>[4x]MPLNRTLSMSSLPGLEDWEDEFDLENAVLFEVAWEVANKVGGIYTVLQTKAKVTGDEWGDNYFLVGPYTEQGVRTQVELLEAPTPALKRTLDSMNSKGCKVYFGRWLIEGGPLVVLLDVGASAWALERWKGELWDTCNIGVPWYDREANDAVLFGFLTTWFLGEFLAQSEEKPHVVAHFHEWLAGVGLCLCRARRLPVATIFTTHATLLGRYLCAGAVDFYNNLENFNVDKEAGERQIYHRYCMERAAAHCAHVFTTVSQITAIEAQHLLKRKP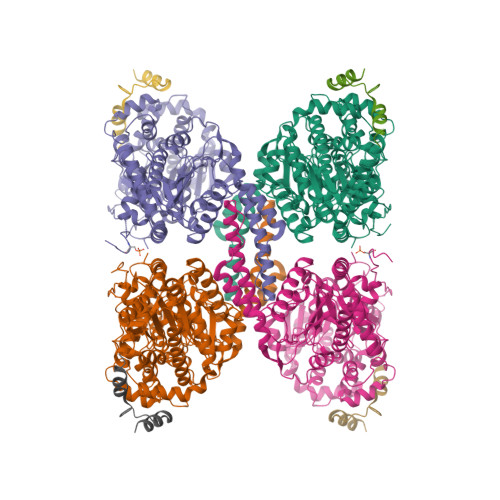DIVTPNGLNVKKFSAMHEFQNLHAQSKARIQEFVRGHFYGHLDFNLDKTLYFFIAGRYEFSNKGADVFLEALARLNYLLRVNGSEQTVVAFFIMPARTNNFNVETLKGQAVRKQLWDTANTVKEKFGRKLYESLLVGSLPDMNKMLDKEDFTMMKRAIFATQRQSFPPVCTHNMLDDSSDPILTTIRRIGLFNSSADRVKVIFHPEFLSSTSPLLPVDYEEFVRGCHLGVFPSYYEPWGYTPAECTVMGIPSISTNLSGFGCFMEEHIADPSAYGIYILDRRFRSLDDSCSQLTSFLYSFCQQSRRQRIIQRNRTERLSDLLDWKYLGRYYMSARHMALSKAFPEHFTYEPNEADAAQGYRYPRPASVPPSPSLSRHSSPHQSEDEEDPRNGPLEEDGERYDEDEEAAKDRRNIRAPEWPRRASCTSSTSGSKRNSVDTATSSSLSTPSEPLSPTSSLGEERN;>MTDQAFVTLTTNDAYAKGALVLGSSLKQHRTTRRLVVLATPQVSDSMRKVLETVFDEVIMVDVLDSGDSAHLTLMKRPELGVTLTKLHCWSLTQYSKCVFMDADTLVLANIDDLFDREELSAAPDPGWPDCFNSGVFVYQPSVETYNQLLHLASEQGSFDGGDQGILNTFFSSWATTDIRKHLPFIYNLSSISIYSYLPAFKVFGASAKVVHFLGRVKPWNYTYDPKTKSVKSEAHDPNMTHPEFLILWWNIFTTNVLPLLQQFGLVKDTCSYVNVLSDLVYTLAFSCGFCRKEDVSGAISHLSLGEIPAMAQPFVSSEERKERWEQGQADYMGADSFDNIKRKLDTYLQ[4x]>[2x]NRMKLMIVGNTGSGKTTLLQQLMKTKKSDLGMQSATVGI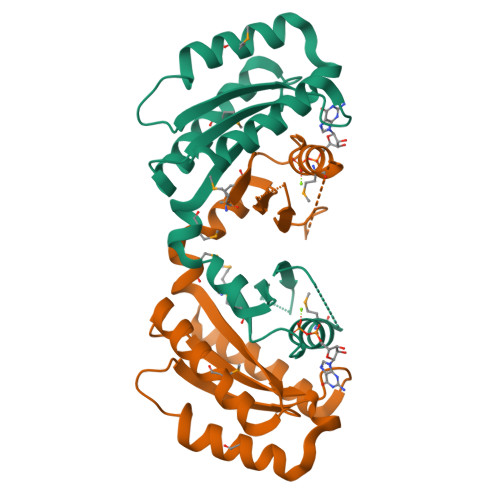DVKDWPIQIRDKRKRDLVLNVWDFAGREEFYSTHPHFMTQRALYLAVYDLSKGQAEVDAMKPWLFNIKARASSSPVILVGTHLDVSDEKQRKACMSKITKELLNKRGFPAIRDYHFVNATEESDALAKLRKTIINESLNFKIRDQ> MPGRRKACFVTALTSRTELDIDPDKLRESVVELLERHPLVFEGTRQLALQHRPEATD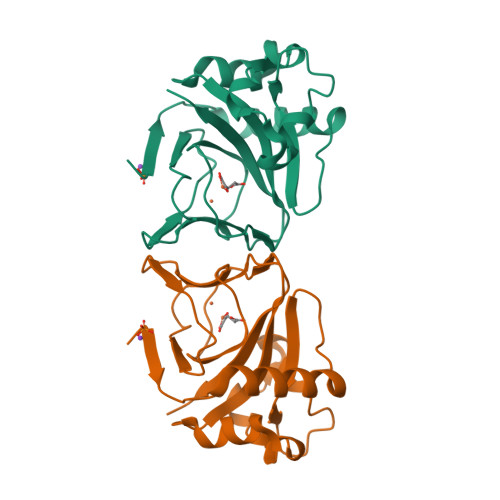PWYEGCQRQSLISSDSDFTEVHGELRDTYLGEVFDRLPFKPIRTRIMALDPKYCYSVHRDLTPRYHLAVTTSEHARFVFIEHDKVLHIPADGDLYYVDTRQLHSAFNGGDDMRIHIVFGTDGESK> MKFTVEREHLLKPLQQVSGPLGGRPTLPILGNLLLQVADGTLSLTGTDLEMEMVARVALVQPHEPGATTVPARKFFDICRGLPEGAEIAVQLEGERMLVRSGRSRFSLSTLPAADFPNLDDWQSEVEFTLPQATMKRLIEATQFSMAHQDVRYYLNGMLFETEGEELRTVATDGHRLAVCSMPIG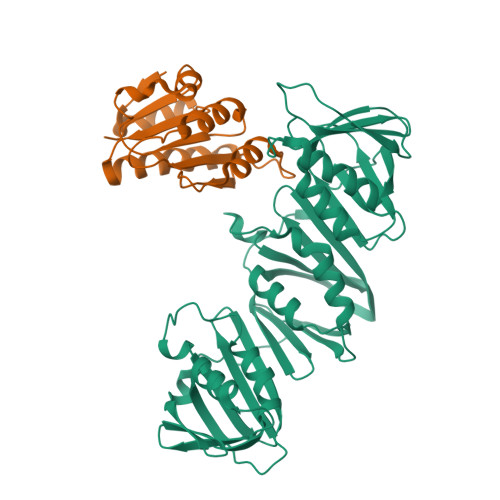QSLPSHSVIVPRKGVIELMRMLDGGDNPLRVQIGSNNIRAHVGDFIFTSKLVDGRFPDYRRVLPKNPDKHLEAGCDLLKQAFARAAAASNEKFRGVRLYVSENQLKITANNPEQEEAEEILDVTYSGAEMEIGFNVSYVLDVLNALKCENVRMMLTDSVSSVQIEDAASQSAAYVVMPMRL;> MIRLYPEQLRAQLNEGLRAAYLLLGNDPLLLQESQDAVRQVAAAQGFEEHHTFSIDPNTDWNAIFSLCQAMSLFASRQTLLLLLPENGPNAAINEQLLTLTGLLHDDLLLIVRGNKLSKAQENAAWFTALANRSVQVTCQ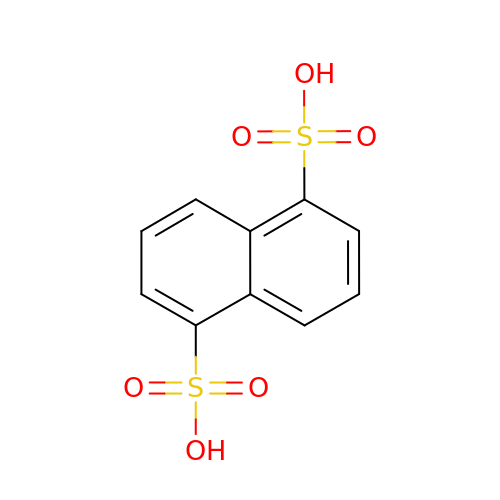naphthalene-1,5-disulfonic acid | C10 H8 O6 S2 | XTEGVFVZDVNBPF-UHFFFAOYSA-N[2-AMINO-3-(4-HYDROXY-PHENYL)-PROPIONYLAMINO]- (2,4,5,8-TETRAHYDROXY-7-OXA-2-AZA-BICYCLO[3.2.1]OCT-3-YL)- 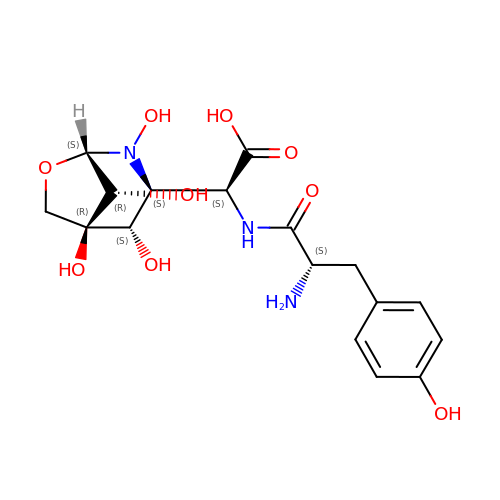ACETIC ACID | C17 H23 N3 O9 | JOBDOAKLPNMGKV-OEUXZGCXSA-N> MN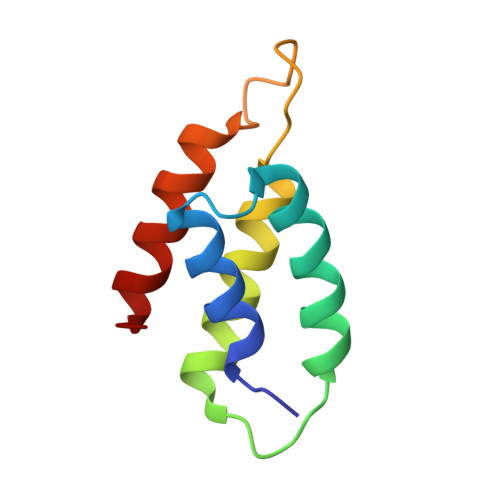KMAMIDLAKLFLASKITAIEFSERICVERRRLYGVKDLSPNILNCGEELFMAAERFEPDADRANYEIDDNGLKVEVRSILEKFKL>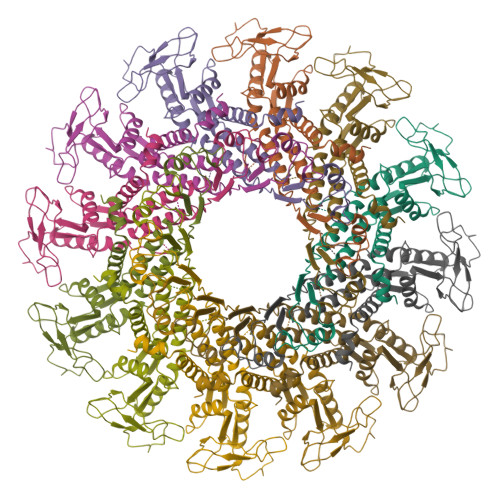[12x]MLEDGFSYKTIGEIQRRRGNLWFRTYQRYLFSLAYQMFEWQGLPKTVDPIFLEKQLHQRGFVAFYKDEMYGYLGVQGTLSGQINLYNQPNFYTASAPTYQKSFPLYWYDMGEDLNEKGQGIVIYNNLERMPTLDILNLYAMNLAELKETIYVNQNAQKTPVIIKAGDNDLFSMKQVYNKYEGNEPVIFAGKKFNTDDIEVLKTDAPYVADKLTMLFKDQWNEAMTFLGLSNANTDKKERLIQSEVESNNDQIQGSANIYLAPRQEACRLINEYYGLNVSVKLRKELVGNGELHNAIEGNSGMGNTV> MVMKLQGVIFDLDGVITDTAHLHFQAWQQIAAEIGISIDAQFNESLKGISRDESLRRILQHGGKEGDFNSQERAQLAYRKNLLYVHSLRELTVNAVLPGIRSLLAD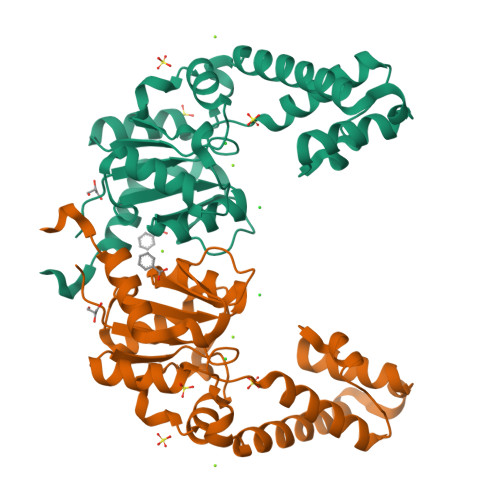LRAQQISVGLASVSLNAPTILAALELREFFTFCADASQLKNSKPDPEIFLAACAGLGVPPQACIGIEDAQAGIDAINASGMRSVGIGAGLTGAQLLLPSTESLTWPRLSAFWQNVAENLYFQSHHHHHHWSHPQFEK The exocyst is an octameric protein complex tethering secretory vesicles to the plasma membrane prior to membrane fusion. The interaction of SAP102 and PSD-95 with the exocyst is via one of its subunits, Sec8, which contains a consensus ITTV motif at the C-terminus for PDZ binding. Previous studies showed that the localization of PSD-95 and SAP102 to neuronal synapses is mediated by the exocyst complex; they together regulate the sorting and trafficking of N-methyl-D-aspartate receptors (NMDARs) from the endoplasmic reticulum (ER) and the Golgi apparatus to the synapse. The complex also plays important roles in cell migration, synaptogenesis, and neurite outgrowth.

We determined a crystal structure for the C-terminal region of Rattus norvegicus Sec8 (aa556–975), which will be called Sec8c hereafter. The crystal belongs to space group I 422 (a = b = 190.004 Å, c = 175.275 Å), with two molecules in the asymmetric unit. One molecule contains aa557–661 and 674–967 of Sec8, and the other contains aa556–662, 675–732, 754–802, 808–936 and 944–967. Except for the flexible loops, the two Sec8 molecules in the asymmetric unit are essentially the same, with an average root-mean-square deviation (RMSD) of approximately 0.5 Å for all aligned backbone atoms. In the structure, we found that the ITTV motif is attached to an enormously long α-helix. The C-terminal half of this helix, which we named “spacer,” protrudes from the helically bundled core of the Sec8 structure. The spacer is sandwiched between the PDZ-binding site and the rest of Sec8. The spacer is slightly shorter in the crystal structure, which was due to the lack of visible electron densities from residue K968 to the C-terminus. Overall, Sec8 is the only exocyst subunit that contains a rigid long spacer that bridges the PDZ-binding ITTV motif to the helical core structure. The results showed no detectable interaction of Sec8c with either PDZ1 or PDZ3, whereas Sec8c bound PDZ2 roubustly, with a Kd of approximately 4 µM.

>HMKTSDPLKILANADTMKVLGVQRPLLQSTIIVEKTVQDLMNLMHDLSAYSDQFLNMVCVKLQEYKDTCSTAYRGIVQSEEKLVISASWAKDDDISRLLKSLPNWTNMAQPKQLRPKREEEEDFIRAAFGKESEVLIGNLGDKLIPPQDILRDVSDLKALANMHESLEWLAGRTKSAFSSLSASQMLSPAQESHVNMDLPPVSEQIMQTLSELAKSFQDMADRCLLVLHLEVRVHCFHYLIPLAKEGNYAIVANVESMDYDPLVVKLNKDISAMEEAMSASLQQHKFQYIFEGLGHLISCILINGAQYFRRISESGIKKMCRNIFVLQQNLTNITMSREADLDFARQYYEMLYNTADELLNLVVDQGVKYTELEYIHALTLLHRSQTGVGDQTTQNTRLQRLKEIICEQAAIKQATKDKKITTV[2x]>MELKNSISDYTEAEFVQLLKEIEKENVAATDDVLDVLLEHFVKITEHPDGTDLIYYPSDNRDDSPEGIVKEIKEWRAANGKPGFKQG[2x];>KRNKPGKATGKGKPVNNKWLNNAGKDLGSPVPDRIANKLRDKEFKSFDDFRKKFWEEVSKDPELSKQFSRNNNDR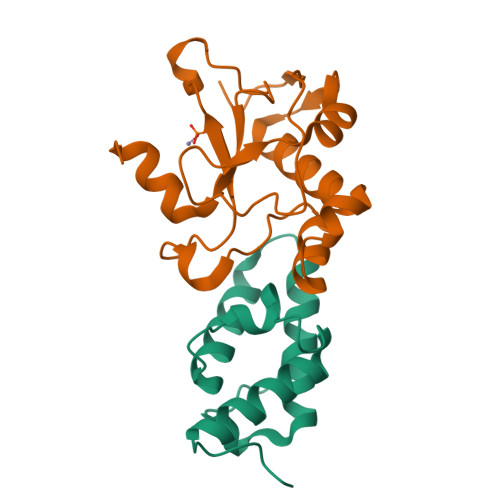MKVGKAPKTRTQDVSGKRTSFELHHEKPISQNGGVYDMDNISVVTPKRHIDIHRGK[2x]> MHFSTLFGAAATAA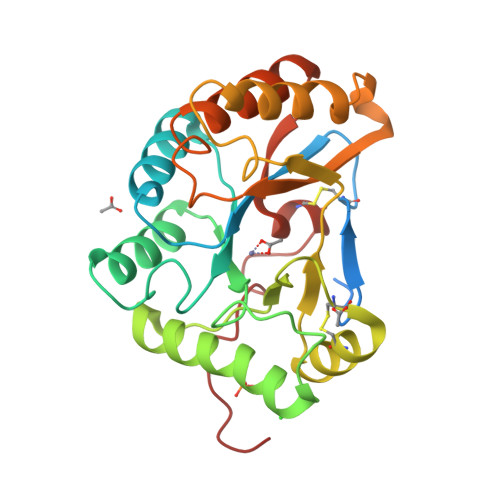LAGSTNASPLARRQVPVGTPILQCTQPGLVALTYDDGPFTFTPQLLDILKQNDVRATFFVNGNNWANIEAGSNPDTIRRMRADGHLVGSHTYAHPDLNTLSSADRISQMRQLEEATRRIDGFAPKYMRAPYLSCDAGCQGDLGGLGYHIIDTNLDTKDYENNKPETTHLSAEKFNNELSADVGANSYIVLSHDVHEQTVVSLTQKLIDTLKSKGYRAVTVGECLGDAPENWYKAHHHHHH(2R)-4-{4-[4-(benzyloxy)-2-fluorophenyl]-2-oxopyridin-1(2H)-yl}-N-hydroxy-2-methyl-2-(methylsulfonyl)butanamide 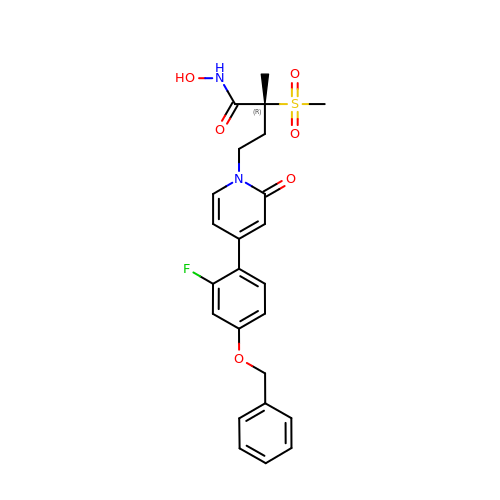| C24 H25 F N2 O6 S | RPIBMYVEZQVKQW-XMMPIXPASA-N>[2x]MQRREFLKLSALGVGAMALRGSGPAKALKAPWYAQEVKSVYQICEGCFWRCGIVAHAVGNRVYKVEGYEANPKSRGRLCPRGQGAPQTTYDPDRLKRPLIRVEGSQRGEGKYRVATWEEALDHIAKKMLEIREKYGPEAIAFFGHGTGDYWFVDFLPAAWGSPNAAKPSVSLCTAPREVASQWVFGRPIGGHEPIDWENARYIVLIGHHIGEDTHNTQLQDFALALKNGAKVVVVDPRFSTAAAKAHRWLPIKPGTDTALLLAWIHVLIYEDLYDKEYVAKYTVGFEELKAHVKDFTPEWAEKHTEIPAQVIREVAREMAAHKPRAVLPPTRHNVWYGDDTYRVMALLYVNVLLGNYGRPGGFYIAQSPYLEKYPLPPLPLEPAAGGCSGPSGGDHEPEGFKPRADKGKFFARSTAIQELIEPMITGEPYPIKGLFAYGINLFHSIPNVPRTKEALKNLDLYVAIDVLPQEHVMWADVILPEATYLERYDDFVLVAHKTPFIQLRTPAHEPLFDTKPGWWIARELGLRLGLEQYFPWKTIEEYLETRLQSLGLDLETMKGMGTLVQR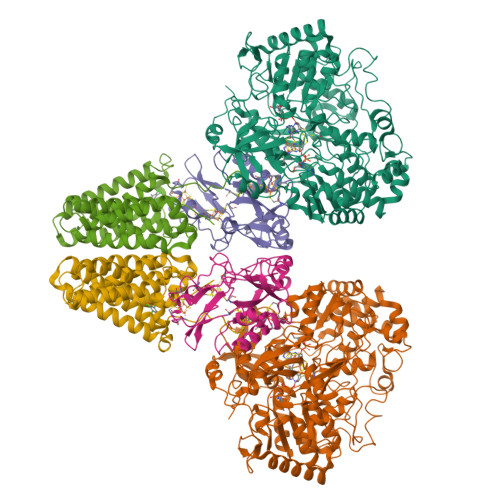GKPWLEDWEKEGRLPFGTASGKIELYCQRFKEAGHQPLPVFTPPEEPPEGFYRLLYGRSPVHTFARTQNNWVLMEMDPENEVWIHKEEAKRLGLKEGDYVMLVNQDGVKEGPVRVKPTARIRKDCVYIVHGFGHKAPLMRLAHGRGASDNYLQTRYKLDPISGGAGLRVNFVRLEKAERPRLPSLTGLAKRPFDERRM;>MPRYAMAIDLSLCVGCAACAVACKMENEVPPGVFNLWIREREVGEYPNLVVEFRPEQCLHCENPPCVPVCPTGASYQTKDGLVLVDPKKCIACGACIAACPYDARYLHPAGYVSKCTFCAHRLEKGKVPACVETCPTYCRTFGDLEDPESPVAKALKAAERVDVLRPEQGTRPKLFYLNAPSKKGLTRESEVHHG[2x];>[2x]MAEFYGLPNAQEFWHWTNALHFVLVGLAGGVALLAALLHLKGDAEARRYTLYALMLIALDLFILWAESPARFRFTHIWLFLSFHPTSPIWWGAWGLGLGFLTGGLLYLGKGSQRALAWALLVFSLVALSYPGLALAVNLNRPLWNGLMAGLFPLTALVLALGLAALLKSPWALFPLRVLAGASLLLALLYPLTLPPEARGHLLEEAGFWYGLFLLLGLGTFWQERLAPWAGLLAAAGLRALLVLAGQWQGLGL>[4x]GSREGCASRCMKY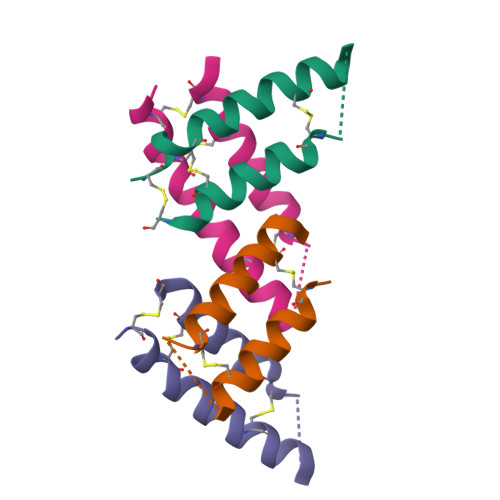NDELEKCEARMMSMSNTEEDCEQELEDLLYCLDHCHSQ> MVKTRSV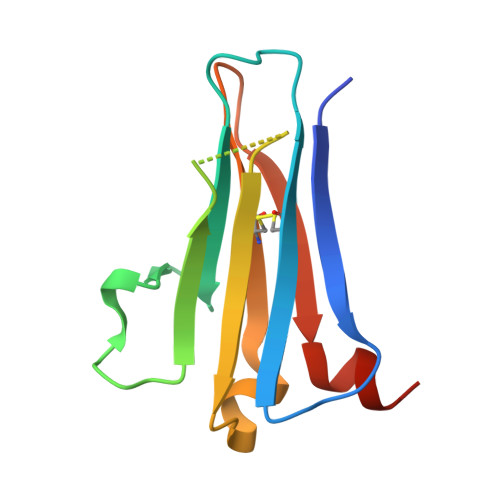NIHVPVKETSKVVLECRGDSYFRHFSYVYWIIGKNKTVDQLPPNSGYRERIYLFKKPHRSENRPRADLILTNITDEMRNEKLTCVLIDPKDPLKESVILSKIWNSVYKI>[2x]AAAAAAMTMMDMNFKYCHKIMKKHSKSFSYAADLLPEDQRKAVWAIYAVCRKIDDSIDVYGDIQFLNQIKEDIQSIEKYPYEYHHFQSDRRIMMALQHVAQHKNIAFQSFYNLIDTVYKDQHFTMFETDAELFGYCYGVAGTVGEVLTPILSDHETHQTYDVARRLGESLQLINILRDVGEDFENERIYFSKQ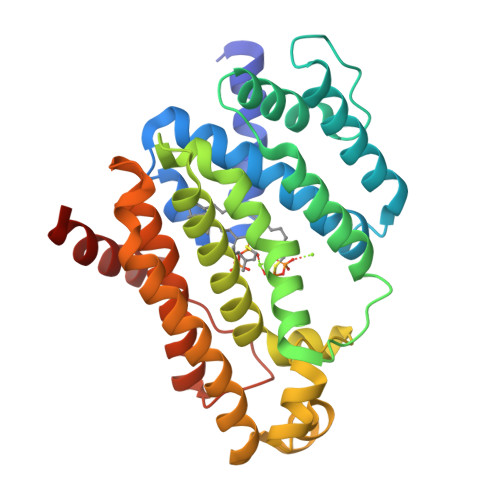RLKQYEVDIAEVYQNGVNNHYIDLWEYYAAIAEKDFRDVMDQIKVFSIEAQPIIELAARIYIEILDEVRQANYTLHERVFVEKRKKAKLFHEINSKYHRI>[2x]MGVPALFRWLSRKYPKIISPVIQDEDVDIDGESRPTRYEDPNPNGELDNLYLDMNGIVHPCSHPEHKPVPETEDEMMLDVFAYTENVIMMARPRKV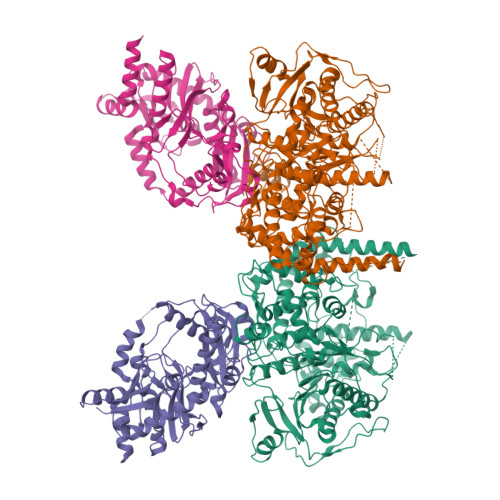IYIAVDGVAPRAKMNQQRSRRFRSAQDAKDANEKKAAELKEMEKKGEIIDDAIKNKKTWDSNAITPGTPFMHRLADSLRYWAAYKLTTDPGWSGIEVIISDASVPGEGEHKIMSYVRSLRSSPKHDPNTTHCIYGLAAALIFLGLATHEPHFKILREDVFAQDKKSYSLQDQLRMTDIERQELKDKKTPFLWLHLNILREYLQIELNVPGLSFPFDLEKSIDDWVFICFFCGNDFLPHLPSLDVRDNSITTLVTIWKQILPTMKGYLTTDGYLNLPAVERLLAELAKKEDYIFRKRYEDEKRSLENQKRRKLAQEQSSARSQNAPNISTGKDKAPLTPNQNIPLYTTSGESVGIKMTDSEMVNNSALITKANEANKSIAELLKQNLQNEINKKRKISNEEQEVVKESVEEVVEEEDDVLVTSDPEDSSTEILIPKNEEIRLWEPGYRKRYYETKFHTKDPQKVKKIARNMVQKYIEGVSWVLLYYYQGCPSWNWYYPYHYAPFAADFVNLSELKIEFVEGTPFRPYEQLMSVLPAASSHNLPDVFRSLMSDANSEIIDFYPEEFPLDMNGKKVIWQAIPLLPFIDENRLLKAVQSKYDQLTEDEKFRNTNRSEILVLGRSHSHYPTLVKELYEEGKDSYEFQVDSSGVSGVAIKLQSFDRSGVLRLPVKQLEGYRHYPDISNRDFLMVEFKQLPKSHAKSMILSGLIPHLRRLTQEDKDSILYGGTNFYGRNRFSPEENADFKQYIGPHGKSQYLPRQGGYKAFIQIHSDEAKGHRHGIYHGGSHTETEFRRGGGYHQHGNRGGRGGYQGNQGYQANSGGYQNSYQGSYQGGYRGGYQGGSQGRYQAGYQSGYQGGYQGEYKNGYQGGYQGNQGNQGYNRQTYNASKSGTLPMKRRHNSGPSSGLEVLFQ;>[2x]GPGMSKEKILPLAARSKKAMLRQPKQVAYFSRDLNYKTHPDRSNLSYYYLPDGDIDNSIDLSVGSKHFLLGDSVELSKLDPILLALKEIEKESGAKTKDRIITWRGIMRKLLTLPYDSEEDFVLDVVSFDGQLFIQFNVPYLKSKDVQKQGDTEFHKKLQFSGYKFEKMATLPKPWPECTRKEIDSRAKSKCNNIEQYGAIVRTGISRIKILIGGAVACTADYYDENDPLSRYIELKTTRTINQYKDMIAFEKKLFRTWAQCFLLGIPKIIYGFRDDNCILRTVEEFSTNDIPLMVKNNPLNEQPKKENCYMSSINFYGAVVEWLNESVKDDQVWKLSYAKRNRQYLVLKEVTDENEKQQIVDSAIPAWFKEWRSELRNSEGNI>MAHHHHHHMKTTPGPVMLDVVGTTLSRDDARRLAHPNTGGVILFARHFQNRAQLTALTDSIRAVREDILIAVDHEGGRVQRFRTDGFTVLPAMRRLGELWDRDVLLATKVATAVGYILAAELRACGIDMSFTPVLDLDYGHSKVIGDRAFHRDPRVVTLLAKSLNHGLSLAGMANCGKHFPGHGFAEADSHVALPT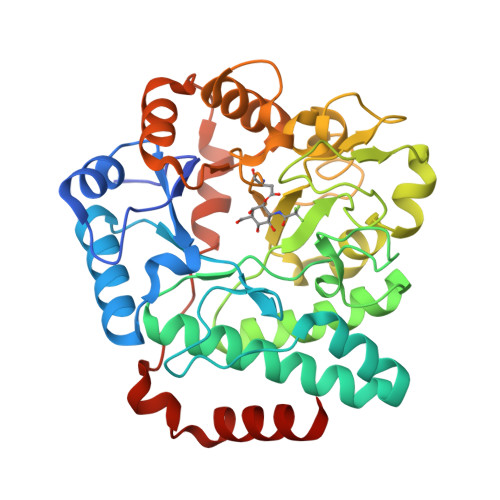DDRTLDAILEQDVAPYDWLGLSLAAVIPAHVIYTQVDKRPAGFSRVWLQDILRGKLGFTGAIFSDDLSMEAAREGGTLTQAADAALAAGCDMVLVCNQPDAAEVVLNGLKARASAESVRRIKRMRARGKALKWDKLIAQPEYLQAQALLSSALA[2x]The unc-51-like kinase protein kinase complex (ULK1C) and the class III phosphatidylinositol (PI) 3-kinase complex I (PI3KC3-C1) are the most upstream and central players in the initiation of macroautophagy. FIP200 is the central scaffolding subunit of the ULK1 complex (ULK1C), which also contains the ULK1 (or ULK2) kinase itself, ATG13, and ATG101. PI3KC3-C1 contains one copy each of the lipid kinase VPS34, the pseudokinase VPS15, and the regulatory subunits BECN1 and ATG14. The two complexes coassemble through extensive contacts between the FIP200 scaffold subunit of ULK1C and the VPS15 pseudokinase subunit of PI3KC3-C1.

Three potential binding sites (#1(370-387), #2(392-398), #3(409-414)) on the opposite side of the ULK1^MIT^ binding and one (#4(449-460)) on the same side of ULK1^MIT^ were identified ([Fig fig2]), consistent with previous hydrogen-deuterium exchange-mass spectrometry (HDX-MS) and site-directed mutagenesis data. The supercomplex structure showed that the N-terminus of the BECN1 and ATG14L binds near ATG13 sites #1-3 on FIP200. The interaction with site #2 is asymmetric and we therefore hypothesized that its main role is to inhibit 2:2:2 ULK1C formation. We hypothesized that PI3KC3-C1 acts by displacing the ATG13 from site #2, and potentially, sites #1 and 3. To test this model, we truncated ATG13^MR^ at residue 450 and determined the structure of the ATG13^1′1–450^ ULK1C core by cryo-EM in the absence of PI3KC3-C1. The 2D averages clearly show densities ULK1^MIT^-ATG13^MIM^ heterodimer on both sides of the shoulder ([Fig fig5]), which was confirmed by 3D reconstruction at 4.46 Å ([Fig figs2]). This demonstrated that ATG13^MR^ has an inhibitory function on recruitment of the second ULK1 kinase to the FIP200 dimer, which is relieved upon formation of the supercomplex with PI3KC3-C1.

>MKLYVFLVNTGTTLTFDTELTVQTVADLKHAIQSKYKIAIQHQVLVVNGGECMAADRRVCTYSAGTDTNPIFLFNKEMILCDRPPAIPKTTFSTENDMEIKVEESLMMPAVFHTVASRTQLALEMYEVAKKLCSFCEGLVHDEHLQHQGWAAIMANLEDCSNSYQKLLFKFESIYSNYLQSIEDIKLKLTHLGTAVSVMAKIPLLECLTRHSYRECLGRLDSLPEHEDSEKAEMKRSTELVLSPDMPRTTNESLLTSFPKSVEHVSPDTADAESGKEIRESCQSTVHQQDETTIDTKDGDLPFFNVSLLDWINVQDRPNDVESLVRKCFDSMSRLDPRIIRPFIAECRQTIAKLDNQNMKAIKGLEDRLYALDQMIASCGRLVNEQKELAQGFLANQKRAENLKDASVLPDLCLSHANQLMIMLQNHRKLLDIKQKCTTAKQELANNLHVRLKWCCFVMLHADQDGEKLQALLRLVIELLERVKIVEALSTVPQMYCLAVVEVVRRKMFIKHYREWAGALVKDGKRLYEAEKSKRESFGKLFRKSFLRNRLFRGLDSWPPSFCTQKPRKFDCELPDISLKDLQFLQSFCPSEVQPFLRVPLLCDFEPLHQHVLALHNLVKAAQSLDEMSQTITDLLSEQK[2x];>[2x]MEQEHTEILRGLRFTLLFVQHVLEIAALKGSASEAAGGPEYQLQESVVADQISLLSREWGFAEQLVLYLKVAELLSSGLQSAIDQIRAGKLCLSSTVKQVVRRLNELYKASVVSCQGLSLRLQRFFLDKQRLLDRIHSITAERLIFSHAVQMVQSAALDEMFQHREGCVPRYHKALLLLEGLQHMLSDQADIENVTKCKLCIERRLSALLTGICA;>[2x]KPAFSKDDILPMDLGTFYREFQNPPQLSSLSIDIGAQSMAEDLDSLPEKLAVHEKNVREFDAFVETLQGSDEA Centrioles are complex microtubule (MT) based structures that are required for the formation of centrosomes and cilia/flagella. The protein kinase recruits STIL/Ana2/SAS-5 and Sas-6 to a single site on the side of the mother centriole where they assemble with CPAP/Sas-4 into a cartwheel structure that helps to establish the ninefold symmetry of the centriole. Here we show that Ana2/STIL proteins also homo-oligomerise and that mutations that perturb the homo-oligomerisation of fly Ana2 in vitro also strongly perturb centriole assembly in vivo. Thus, Sas-6 homo-oligomerisation alone appears unable to drive efficient cartwheel assembly in vivo if Ana2 is unable to homo-oligomerise.

In initial attempts to purify Sas-61–241 the protein invariably formed large aggregates (blue trace) that appeared to be elongated chains of protein by negative-stain EM (Figure 6Ci–iv). It has previously been shown that a large hydrophobic residue in the headgroup is essential for the N–N interaction in several species, so we mutated the equivalent residue, F143, to Asp. Purified Sas-61–241-F143D behaved as a dimer by SEC-MALS (red trace) and aggregates were no longer detectable by negative-stain EM; we conclude that aggregate formation is dependent upon the N–N interaction, and the F143D mutation perturbs this interaction in vitro. To investigate how Drosophila Sas-6 might oligomerise into a cartwheel we solved the crystal structure of Sas-61–216-F143D to 2.9 Å. The asymmetric unit contained a dimer of Sas-6, associated via the coiled-coil interface. The DmSas-6 N-CC dimer could be superimposed with Sas-6 N-CC dimers from D. rerio, Chlamydomonas and Leishmania Sas-6 (average pairwise RMSD 1.87 ± 0.31 Å over 617 ± 47 backbone atom pairs). However it could not be superimposed onto C. elegans SAS-6, which has an alternative head-group-spoke conformation. Furthermore, we found that the DmSas-6 N-CC dimer could be modelled into a flat ninefold ring, similar to that observed in crystallo for Leishmania Sas-6. We also examined the structure of Drosophila Sas-6 and confirmed that, similar to other Sas-6 orthologues, it associates via two self-interaction interfaces, a C-terminal coiled-coil dimerization (C–C), and an N-terminal headgroup oligomerization (N–N). The interface between the headgroup and the C–C was similar to that seen in most other species, and different to that observed in C. elegans strongly suggesting that Drosophila Sas-6 assembles into a canonical, flat ring structure. In agreement with previous studies, we found that mutations that perturb the ability of Drosophila Sas-6 to homo-oligomerise through the N–N interface in vitro (GFP-Sas-6-F143D) cannot support efficient centriole duplication in vivo, and this is also true for mutations that perturb the ability of Ana2 to tetramerise in vitro (Ana2-CCA-GFP).

>GPMGWPPGSEDSYSAKMDYGKSVVNILPSVEMLVNFNGDMTRSSKRSCLLYAERVDFKELLQLRLTEKSDQRRMYITTVDSASFQDLKQDQSLNVSFSGFIDNVVRMLKDCQSGKLELHLTTRDQNLSSGREVHDYYLQFVEIRSDKNLVHLSLPCRSAPLNTVLFYINSMLEASHKKQYILEQSMQQMQAEINAQRAHAERLTTENTNLREALAENTR[2x]>[2x]MPLNPHVEALLQMMAQMPAPDFSVANPAEIRAVFDNLAAPPQVARVENIAISLDGRDLDARLYVPEDADERPALMVYYHGGGWVIGTLDTHDGTCRALAQKSGCAVLSIAYRLAPEYRYPAPAEDCYDALVWAKQNAATLGVDGDRLAVGGDSAGGNLAAAVAIMARDRNGPALRHQLLIYPVTDNDFTLASYAENGGGEYYLSTDGMRWFWGHYLGDTAAENAPLAAVLNVADLSGLAPATVI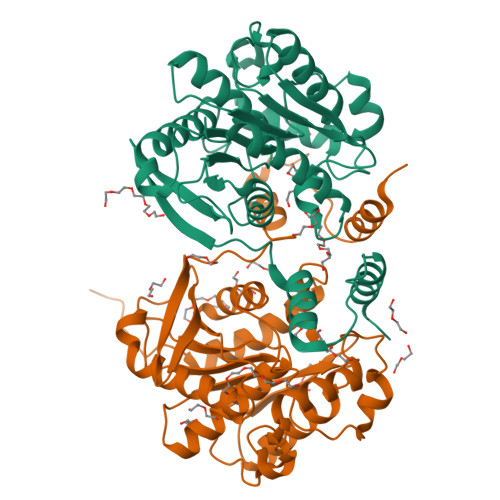TAEYDPLRDEGIAYAKKLDAAGVPVDAATAPGMIHGFFSMFEAVPDSWEWIERGASNLKRDLALEHHHHHHHH3-[1-[3-[(4~{S})-6-azanyl-5-cyano-3-methyl-4-propan-2-yl-2~{H}-pyrano[2,3-c]pyrazol-4-yl]-5-fluoranyl-phenyl]piperidin-4-yl]propanoic acid | C25 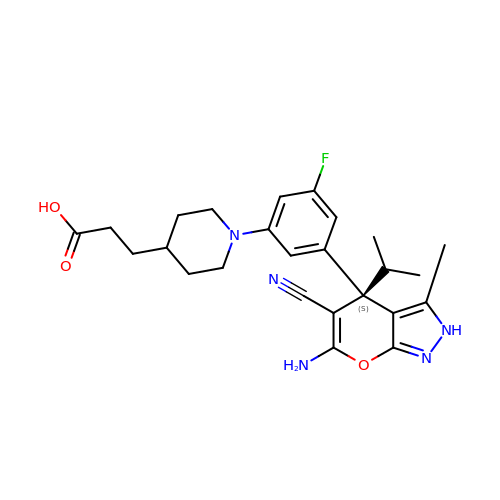H30 F N5 O3 | MARQRCANXIMJDC-VWLOTQADSA-N>MTQGAVKTTGKRSRAVSAKKKAILSAALDTFSQFGFHGTRLE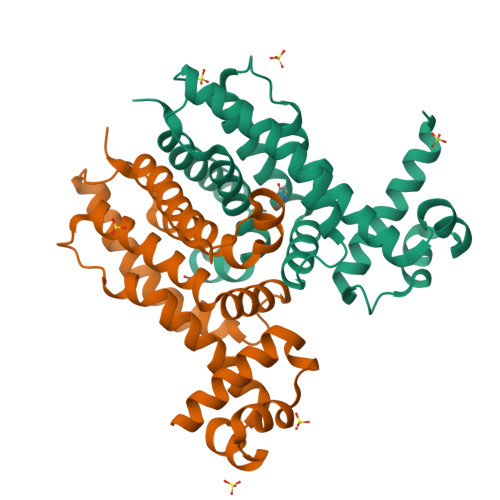QIAELAGVSKTNLLYYFPSKEALYIAVLRQILDIWLAPLKAFREDFAPLAAIKEYIRLKLEVSRDYPQASRLFCMEMLAGAPLLMDELTGDLKALIDEKSALIAGWVKSGKLAPIDPQHLIFMIWASTQHYADFAPQVEAVTGATLRDEVFFNQTVENVQRIIIEGIRPR[2x]> QINFYKDSYAASASK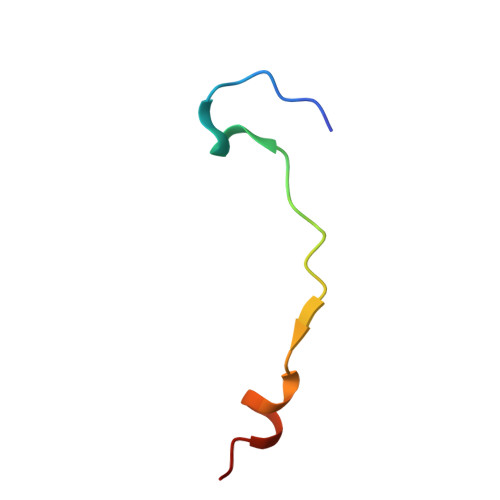QDFSQDPSKFTEPVV>[2x]GSGNSHTTPWTNPGLAENFMNSFMQGLSSMPGFTASQLDDMSTIAQSMVQSIQSLAAQGRTSPNKLQALNMAFASSMAQIAASEEGGGSLSTKTSSIASAMSN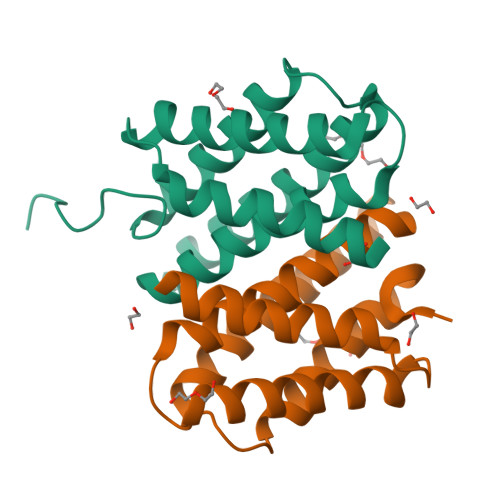AFLQTTGVVNQPFINEITQLVSMFAQAGMNDVSA> MSRESNDTIQSDTVRSSSKSDYFRIQLNNQDYYMSKPTFLDPSHGESLPLNQFSQVPNIRVFGALPTGHQVLCHVHGILPYMFIKYDGQITDTSTLRHQRCAQVHKTLEVKIRASFKRKKDDKHDLAGDKLGNLNFVADVSVVKGIPFYGYHVGWNLFYKISLLNPSCLSRISELIRDGKIFGKKFEIYESHIPYLLQWTADFNLFGCSWINVDRCYFRSPVLNSILDIDKLTINDDLQLLLDRFCDFKCNVLSRRDFPRVGNGLIEIDILPQFIKNREKLQHRDIHHDFLEKLGDISDIPVKPYVSSARDMINELTMQREELSLKEYKEPPETKRHVSGHQWQSSGEFEAFYKKAQHKTSTFDGQIPNFENFIDKNQKFSAINTPYEALPQLWPRLPQIEINNNSMQDKKNDDQVNASFTEYEICGVDNENEGVKGSNIKSRSYSWLPESIASPKDSTILLDHQTKYHNTINFSMDCAMTQNMASKRKLRSSVSANKTSLLSRKRKKVMAAGLRYGKRAFVYGEPPFGYQDILNKLEDEGFPKIDYKDPFFSNPVDLENKPYAYAGKRFEISSTHVSTRIPVQFGGETVSVYNKPTFDMFSSWKYALKPPTYDAVQKWYNKVPSMGNKKTESQISMHTPHSKFLYKFASDVSGKQKRKKSSVHDSLTHLTLEIHANTRSDKIPDPAIDEVSMIIWCLEEETFPLDLDIAYEGIMIVHKASEDSTFPTKIQHCINEIPVMFYESEFEMFEALTDLVLLLDPDILSGFEIHNFSWGYIIERCQKIHQFDIVRELARVKCQIKTKLSDTWGYAHSSGIMITGRHMINIWRALRSDVNLTQYTIESAAFNILHKRLPHFSFESLTNMWNAKKSTTELKTVLNYWLSRAQINIQLLRKQDYIARNIEQARLIGIDFHSVYYRGSQFKVESFLIR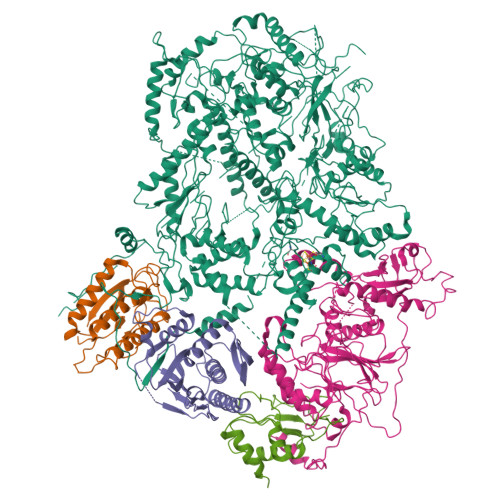ICKSESFILLSPGKKDVRKQKALECVPLVMEPESAFYKSPLIVLDFQSLYPSIMIGYNYCYSTMIGRVREINLTENNLGVSKFSLPRNILALLKNDVTIAPNGVVYAKTSVRKSTLSKMLTDILDVRVMIKKTMNEIGDDNTTLKRLLNNKQLALKLLANVTYGYTSASFSGRMPCSDLADSIVQTGRETLEKAIDIIEKDETWNAKVVYGDTDSLFVYLPGKTAIEAFSIGHAMAERVTQNNPKPIFLKFEKVYHPSILISKKRYVGFSYESPSQTLPIFDAKGIETVRRDGIPAQQKIIEKCIRLLFQTKDLSKIKKYLQNEFFKIQIGKVSAQDFCFAKEVKLGAYKSEKTAPAGAVVVKRRINEDHRAEPQYKERIPYLVVKGKQGQLLRERCVSPEEFLEGENLELDSEYYINKILIPPLDRLFNLIGINVGNWAQEIVKSKRASTTTTKVENITRVGTSATCCNCGEELTKICSLQLCDDCLEKRSTTTLSFLIKKLKRQKEYQTLKTVCRTCSYRYTSDAGIENDHIASKCNSYDCPVFYSRVKAERYLRDNQSVQREEALISLNDW;>MNRWVEKWLRVYLKCYINLILFYRNVYPPQSFDYTTYQSFNLPQFVPINRHPALIDYIEELILDVLSKLTHVYRFSICIINKKNDLCIEKYVLDFSELQHVDKDDQIITETEVFDEFRSSLNSLIMHLEKLPKVNDDTITFEAVINAIELELGHKLDRNRRVDSLEEKAEIERDSNWVKCQEDENLPDNNGFQPPKIKLTSLVGSDVGPLIIHQFSEKLISGDDKILNGVYSQYEEGESIFGSLF[2x];> LHMDALLTKFNEDRSLQDENLSQPRTRVRIVDDNLYNKSNPFQLCYKKRDYGSQYYHIYQYRLKTFRERVLKECDKRWDAGFTLNGQLVLKKDKVLDIQGNQPCWCVGSIYCEMKYKPNVLDEVINDTYGAPDLTKSYTDKEGGSDEIMLEDESGRVLLVGDFIRSTPFITGVVVGILGMEAEAGTFQVLDICYPTPLPQNPFPAPIATCPTRGKIALVSGLNLNNTSPDRLLRLEILREFLMGRINNKIDDISLIGRLLICGNSVDFDIKSVNKDELMISLTEFSKFLHNILPSISVDIMPGTNDPSDKSLPQQPFHKSLFDKSLESYFNGSNKEILNLVTNPYEFSYNGVDVLAVSGKNINDICKYVIPSNDNGESENKVEEGESNDFKDDIEHRLDLMECTMKWQNIAPTAPDTLWCYPYTDKDPFVLDKWPHVYIVANQPYFGTRVVEIGGKNIKIISVPEFSSTGMIILLDLETLEAETVKIDI;> MDQKASYFINEKLFTEVKPVLFTDLIHHLKIGPSMAKKLMFDYYKQTTNAKYNCVVICCYKDQTIKIIHDLSNIPQQDSIIDCFIYAFNPMDSFIPYYDIIDQKDCLTIKNSYELKVSESSKIIERTKTLEEKSKPLVRPTARSKTTPEETTGRKSKSKDMGLRSTALLAKMKKDRDDKETSRQNELRKRKEENLQKINKQNPEREAQMKELNNLFVEDDLDTEEVNGGSKPNSPKETDSNDKDKNNDDLEDLLETTAEDSLMDVPKIQQTKPSETEHSKEPKSEEEPSSFIDEDGYIVTKRPATSTPPRKPSPVVKRALSSSKKQETPSSNKRLKKQGTLESFFKRKAK> MADWVTGKVTKVQNWTDALFSLT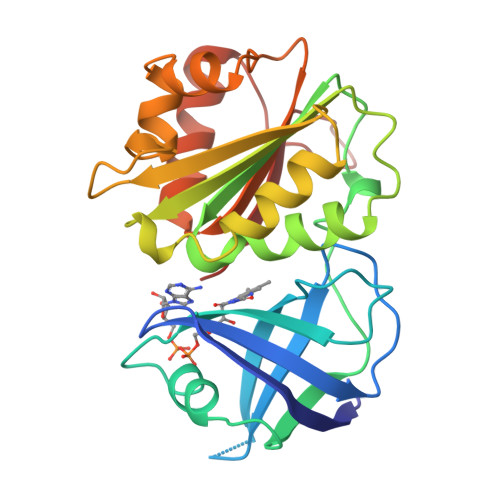VHAPVLPFTAGQFTKLGLEIDGERVQRAYSYVNSPDNPDLEFYLVTVPDGKLSPRLAALKPGDEVQVVSEAAGFFVLDEVPHCETLWMLATGTAIGPYLSILRLGKDLDRFKNLVLVHAARYAADLSYLPLMQELEKRYEGKLRIQTVVSRETAAGSLTGRIPALIESGELESTIGLPMNKETSHVMLCGNPQMVRDTQQLLKETRQMTKHLRRRPGHMTAEHYW>MGLAVFLPPYPFRGLKAPYLWMFYKYLHCATDSILFITGEDYLSVTDDEAQRARWEFDPASMASLGYELPNAQSMACHEYLTLDNAFYETLLSRHHHDPIKSFSAFLTERIPDLETELHALLDSKKGIIDQIDTFISICNCPSLEHVARTLGKEVMHIEIGPLRAPMYRNTAYLDFAGVNGGTEASARYEKCQAEFDIKASLGDLHNYFLEVLPPAEAATHSAAGVVLQVEDDSNLIAYNHDFTNISLLSYVRQR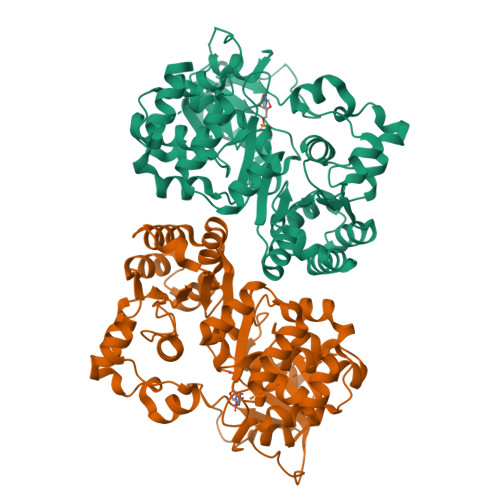YEKEDILVRAHPGSLFRLRDDVFTIDDSANSLAFINQCNEVFTINSSVGLEAILTGKKTTVLGDCSYAFINELAGASATVNAAAFYLFSYLVPFDLVFNQEYLKFRLGHPEEREIVGKHIEFYSADMPGSLSQAAHSLSSLINEAISLEHHHHHH[2x]>[3x]SGKPVLHYFNARGRMECIRFLLAAAGVEFDEKF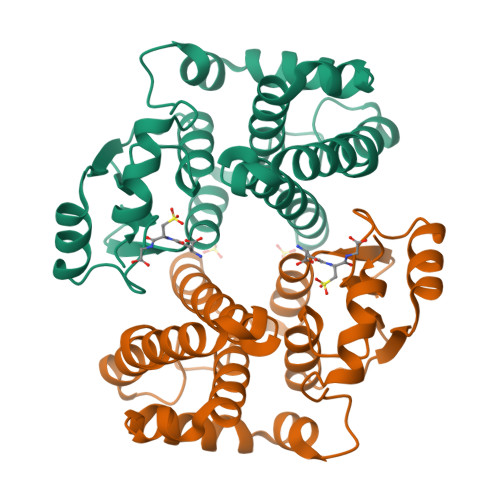IQSPEDLEKLKKDGNLMFDQVPMVEIDGMKLAQTRAILNYIATKYDLYGKDMKERALIDMYSEGILDLTEMIMQLVICPPDQKEAKTALAKDRTKNRYLPAFEKVLKSHGQDYLVGNKLTRVDIHLLELLLYVEEFDASLLTSFPLLKAFKSRISSLPNVKKFLQPGSQRKLPMDAKQIEEARKIYKF> PISPIETVPVKLKPGMDGPKVKQWPLTEEKIKALVEICTEMEKEGKISKIGPENPYNTPVFAIKKKDSTKWRKLVDFRELNKRTQDFWEVQLGIPHPAGLKKKKSVTVLDVGDAYFSVPLDEDFRKYTAFTIPSINNETPGIRYQYNVLPQGWKGSPAIFQSSMTKILEPFRKQNPDIVIYQYMDDLYVGSDLEIGQHRTKIEELRQHLLRWGLTTPDGYELHPDKWTVQPIVLPEKDSWTVNDIQKLVGKLNWASQIYPGIKVRQLSKLLRGTKALTEVIPLTEEAELELAENREILKEPVHGVYYDPSKDLIAEIQKQGQGQWTYQIYQEPFKNLKTGKYARMRGAHTNDVKQLTEAVQKITTESI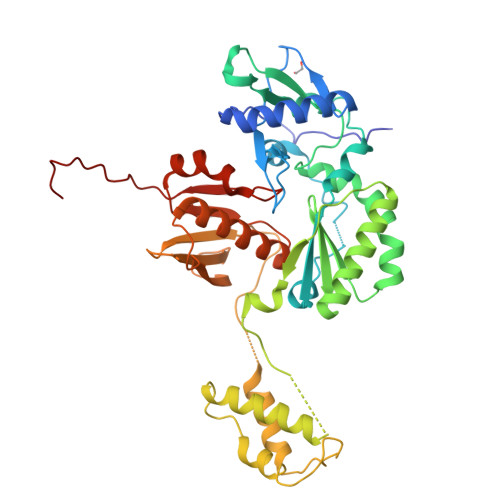VIWGKTPKFKLPIQKETWETWWTEYWQATWIPEWEFVNTPPLVKLWYQLE> MFPAAPSPRTPGTGSRRGPLAGLGPGSTPRTASRKGLPLGSAVSSPVLFSPVGRRSSLSSRGTPTRMFPHHSITESVNYDVKTFGSSLPVKVMEALTLAEVDDQLTINIDEGGWACLVCKEKLIIWKIALSPITKLSVCKELQLPPSDFHWSADLVALSYSSPSGEAHSTQAVAVMVATREGSIRYWPSLAGEDTYTEAFVDSGGDKTYSFLTAVQGGSFILSSSGSQLIRLIPESSGKIHQHILPQGQGMLSGIGRKVSSLFGILSPSSDLTLSSVLWDRERSSFYSLTSSNISKWELDDSSEKHAYSWDINRALKENITDAIWGSESNYEAIKEGVNIRYLDLKQNCDGLVILAAAWHSADNPCLIYYSLITIEDNGCQMSDAVTVEVTQYNP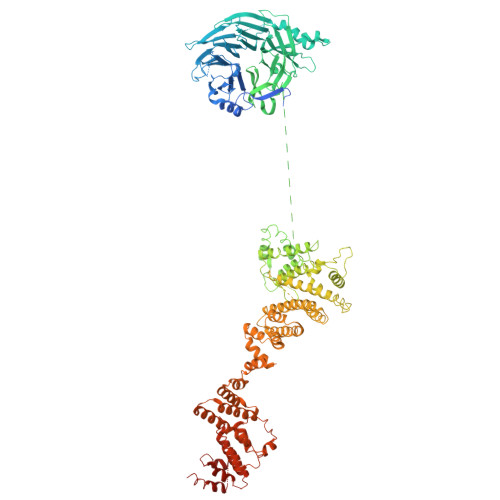PFQSEDLILCQLTVPNFSNQTAYLYNESAVYVCSTGTGKFSLPQEKIVFNAQGDSVLGAGACGGVPIIFSRNSGLVSITSRENVSILAEDLEGSLASSVAGPNSESMIFETTTKNETIAQEDKIKLLKAAFLQYCRKDLGHAQMVVDELFSSHSDLDSDSELDRAVTQISVDLMDDYPASDPRWAESVPEEAPGFSNTSLIILHQLEDKMKAHSFLMDFIHQVGLFGRLGSFPVRGTPMATRLLLCEHAEKLSAAIVLKNHHSRLSDLVNTAILIALNKREYEIPSNLTPADVFFREVSQVDTICECLLEHEEQVLRDAPMDSIEWAEVVINVNNILKDMLQAASHYRQNRNSLYRREESLEKEPEYVPWTATSGPGGIRTVIIRQHEIVLKVAYPQADSNLRNIVTEQLVALIDCFLDGYVSQLKSVDKSSNRERYDNLEMEYLQKRSDLLSPLLSLGQYLWAASLAEKYCDFDILVQMCEQTDNQSRLQRYMTQFADQNFSDFLFRWYLEKGKRGKLLSQPISQHGQLANFLQAHEHLSWLHEINSQELEKAHATLLGLANMETRYFAKKKTLLGLSKLAALASDFSEDMLQEKIEEMAEQERFLLHQETLPEQLLAEKQLNLSAMPVLTAPQLIGLYICEENRRANEYDFKKALDLLEYIDEEEDININDLKLEILCKALQRDNWSSSDGKDDPIEVSKDSIFVKILQKLLKDGIQLSEYLPEVKDLLQADQLGSLKSNPYFEFVLKANYEYYVQGQI>[2x]MPCTEQITLYTTTFSPYGHRAHIALEEAGAEYTLCQINVHRDKPEWYKRVNPLGKVPAITFGGPQVP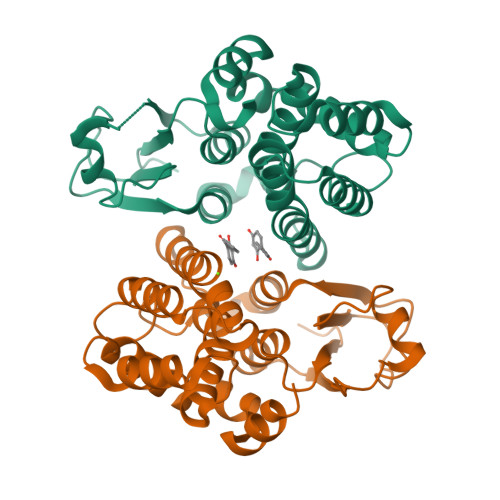PDEPSPESEKLVESLALLEFVADVFPEAKLLPASPVQRARARAFIAIYQNYLHDQFRDAFFRGEPVGPFLQALETLQSALPPAGFAVGEWSLAEAAVAPFLARMMLYLDAGLGKYSEADGETMRAALASERFARISQYVRDIRARASFVKSWGGDDVQLEAAKAIPMLRRPAHHHHHH>TAELKICRVNRNSGSCLGGDEIFLLCDKVQKEDIEVYFTGPGWEARGSFSQADVHRQVAIVFRTPPYADPSLQAPVRVSMQLRRPSDRELSEPMEFQYLPDTDDRHRIEEKRKRTYETFKSIMKKSPFNGPTEPRP[2x];> VFGYVTEDGDTALHLAVIHQHEPFLDFLLGFSAGHEYLDLQNDLGQTALHLAAILGEASTVEKLYAAGAGVLVAERGGHTALHLACRVRAHTCACVLLQPRPSHPRDASDTYLTQSQDCTPDTSHAPAAVDSQPNPENEE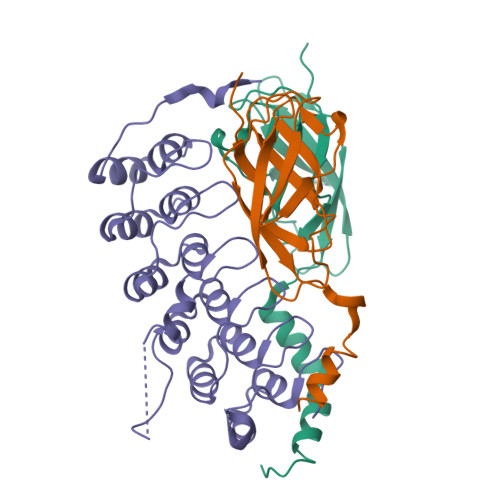EPRDEDWRLQLEAENYDGHTPLHVAVIHKDAEMVRLLRDAGADLNKPEPTCGRTPLHLAVEAQAASVLELLLKAGADPTARMYGGRTPLGSALLRPNPILARLLRAHGAPEPEDGGDKLSPCEEEGEDEDSDNRDEGDEYDD> GPGSSSSSIATTGSQESFV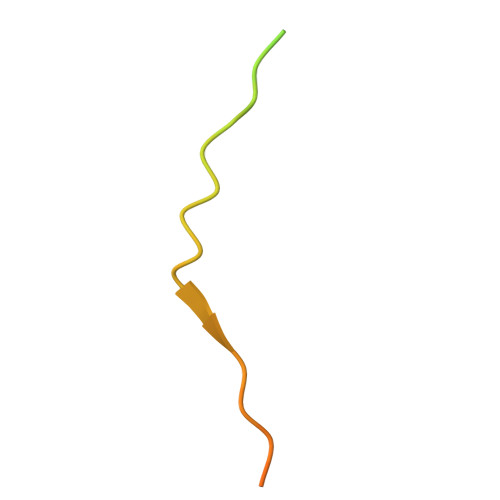ARPFKKGLNLHSIKVTSSTPKGSENLYFQ>[2x]VLSQIAICIWVESTAILQDCQRALSADRYQLQVCESGEMLLEYAQTHRDQIDCLILVAANPSFRAVVQQLCFEGVVVPAIVVGDRDSEDPDEPAKEQLYHSAELHLGIHQLEQLPYQVDAALAEF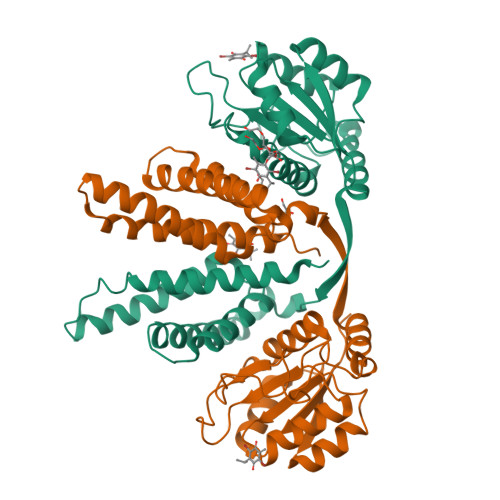LRLAPVETMADHIMLMGANHDPELSSQQRDLAQRLQERLGYLGVYYKRDPDRFLRNLPAYESQKLHQAMQTSYREIVLSYFSPNSNLNQSIDNFVNMAFFADVPVTKVVEIHMELMDEFAKKLRVEGRSEDILLDYRLTLIDVIAHLCEMYRRSIPRET>[2x]MGSSHHHHHHSQDPSSMTMELRPSGDSGSSDVDAEISDGFSPLDTSHRDVADEGSLLRRAEMYQDYMKQVPIPTNRGSLIPFTSWVGLSISMKQLYGQPLHYLTNVLLQRWDQSRFGTDSEEQRLDSIIHPTKAEATIWLVEEIHRLTPSHLHMALLWRSDPMYHSFIDPIFPEK;>[4x]MADLYPTGQQISFQTTPLN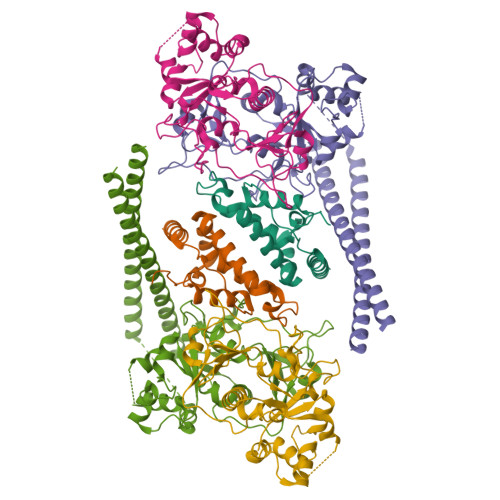VQDPTRMMNLDQSSPVARNETQNGGGIAHAEFAMFNSKRLESDLEAMGNKIKQHEDNLKFLKSQKNKMDEAIVDLQVHMSKLNSSPTPRSENSDNSLQGEDINAQILRHENSAAGVLSLVETLHGAQASQLMLTKGVVGVVAKLGKVNDENLSQILSNYLGTRSMLAVVCRNYESVTALEAYDNHGNIDINAGLHCLGSSIGREIGDSFDAICLENLRPYVGQHIADDLQRRLDLLKPKLPNGECPPGFLGFAVNMIQIDPAYLLCVTSYGYGLRETLFYNLFSRLQVYKTRADMISALPCISDGAVSLDGGIIRKTGIFNLGNRDEVNVRFAKPTASRTMDNYSEAEKKMKELKWKKEKTLEDIKREQVLREHAVFNFGKKKEEFVRCLAQSSCTNQPMNTPRGTLESGKETAAAKFERQHMDSSTSAA>MEKVPGEMEIERRERSEELSEAERKAVQAMWARLYANSEDVGVAILVRFFVNFPSAKQYFSQFKHMEDPLEMERSPQLRKQASRVMGALNTVVENLHDPDKVSSVLALVGKAHALKHKVEPVYFKILSGVILEVVAEEFASDFPPETQRAWAKLRGLIYSHVTAAYKEVGWVQQVPNATTPPATLPSSGP[2x]

Almost independently, the sequence of this globin was identified in mouse, man and zebrafish and, given that it is expressed in all types of human tissues, was eventually termed cytoglobin (Cygb). Human Cygb consists of 190 amino acids, showing extensions of about 20 amino acids at both C- and N-termini with respect to standard globins. In the absence of exogenous ligands, the sixth heme iron coordination position is occupied by the distal HisE7 residue in both the ferric and ferrous forms.

Since the HE7Q mutation disrupts the endogenous bis-histidyl hexacoordination with HisE7, the comparison of wt Cygb* and its HE7Q mutant provides clues on the transition from exogenous hexacoordination to the endogenous one through the pentacoordinated species. The two subunits (A, B) found in the X-ray structure are assembled in a dimer identical to that found for native Cygb*. Superimposition of the Cα atoms in the protein core of the two subunits reveals a strong structural conservation (rmsd of 0.45 Å), with limited differences in the G-H loop (residues 137–146). The cyanide ligand in the distal site pocket is found almost parallel to the heme plane (distance of 3.22 and 2.87 Å found in subunits A and B of the X-ray structure), oriented roughly along the line connecting the pyrrole NA and NC nitrogen atoms. This arrangement indicates that the structure better fits a pentacoordinated protein. The absence of ligand coordination likely arises from X-ray-induced Fe(III)→Fe(II) reduction, resulting essentially in loss of heme affinity for the ligand, as has been noticed for other heme proteins. Structural overlays of the HE7Q mutant with bis-histidyl hexa- (subunit A) and pentacoordinated (subunit B) Cygb* yield a rmsd of 0.66 Å and 0.51 Å, respectively. The largest deviations are found at residues 60–66 and 70–83 (CD-D stretch and beginning of helix E), as the shift from endogenous bis-histidyl hexacoordination to pentacoordination drives the E-helix 1.5 Å away from the distal site pocket (measured on the Cα atom of the E7 residue), increasing the distal site volume by about 73 Å3. In the HE7Q mutant the Gln side-chain matches the position of His in the pentacoordinated structure, as the side chain amide N atom is shifted only ∼1 Å relative to the His Nε atom. However, the Gln side chain is pointing to the exterior of the distal site, while the His side chain is oriented to the interior, thus suggesting that the pentacoordinated native Cygb* highlights an intermediate position of HisE7 in the mechanism controlling exogenous ligand binding through competition with the endogenous ligand.>MGHHHHHHMSDKFSHITKDITTQLAKFRKEMPELMTGFSSLAQAATKDGALDKKTKELIAMALAVAKQCPGCIGFHSQTLVKLQATREELLETLGMAVYMGGGPSLMYAAEALEAF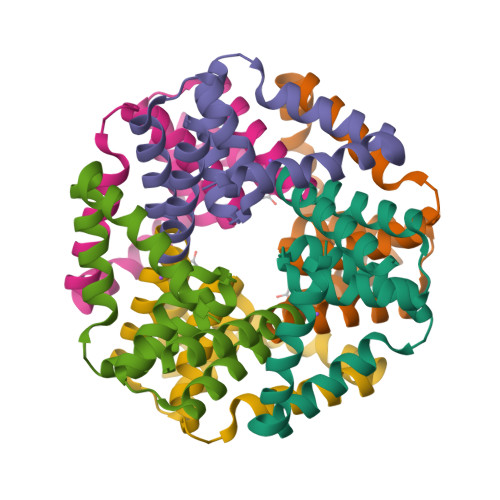EEFSK[2x]>[2x]MINQNATYMEESAQSAVDNFGLGFNLGNTLDANGCGTGKPVATYETFWGQPETTQDMMTFLMQNGFNAV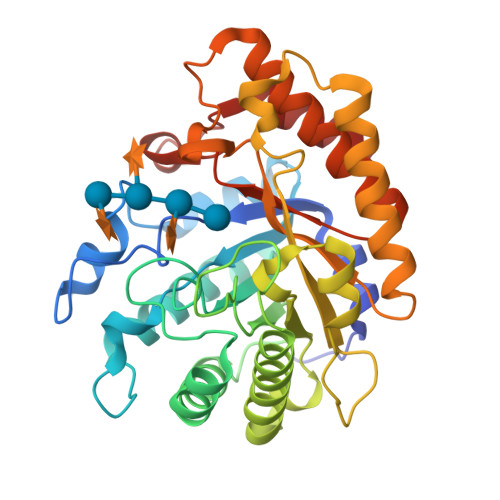RIPVTWYEHMDAEGNVDEAWMMRVKAIVEYAMNAGLYAIVNVHHDTAAGSGAWIKADTDVYAATKEKFKKLWTQIANALADYDQHLLFEGYNEMLDGNNSWDEPQKASGYEALNNYAQDFVDAVRATGGNNATRNLIVNTYAAAKGENVLNNFMLPTDAVNNHLIVQVHSYDPWNFFNTKTTWDSECHNTLTEIFSALSKKFTTIPYIIGAYGTHGESDISVSKSSPAEKIKLAADQAADMVKLAKDHHSATFYWMSIFDGSDRIQPQWSLPTVVEAMQEAYNN>[2x]GPNPQTEEVSIKEIAITHHVKEGHEKADPSQFELLKVLGQGSFGKVFLVKKISGSDARQLYAMKVLKKATLKVRDRVRTKMERDILVEVNHPFIVKLHYAFQTEGKLYLILDFLRGGDLFTRLSKEVMFTEEDVKFYLAELALALDHLHSLGIIYRDLKPENILLDEEGHIKLTD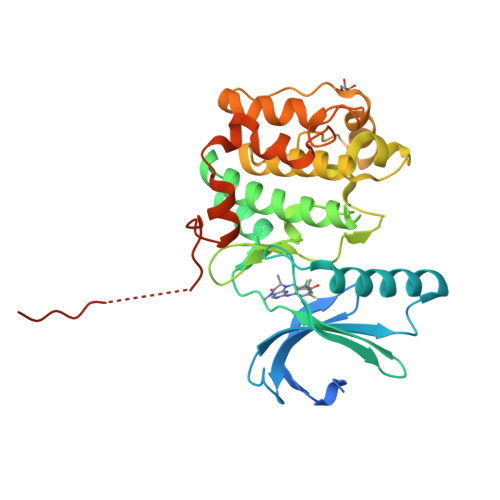FGLSKESIDHEKKAYSFCGTVEYMAPEVVNRRGHTQSADWWSFGVLMFEMLTGTLPFQGKDRKETMTMILKAKLGMPQFLSPEAQSLLRMLFKRNPANRLGAGPDGVEEIKRHSFFSTIDWNKLYRREIHPPFKPATGRPEDTFYFDPEFTAKTP>MSLYNYVLFDLDGTLTDSAEGITKSVKYSLNKFDIQVEDLSSLNKFVGPPLKTSFMEYYNFDEETATVAIDYYRDYFKAKGMFENKVYDGIEALLSSLKDYGFHLVVATSKPTVFSKQILEHFKLAFYFDAIVGSSLDGKLSTKEDVIRYAMESLNIK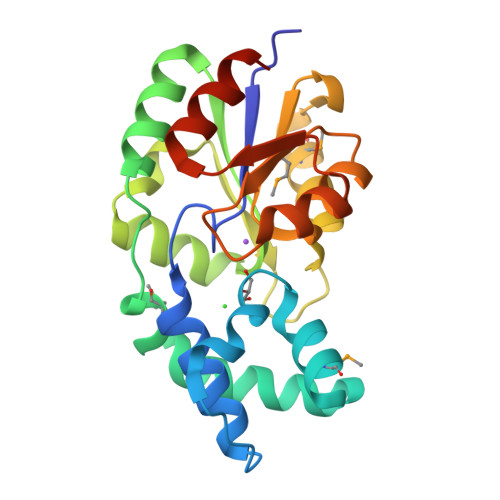SDDAIMIGDREYDVIGALKNNLPSIGVTYGFGSYEELKNAGANYIVNSVDELHKKILELREGHHHHHH[2x]N-(6-cyano-3-{2-[2-(2,4-dioxo-3,4-dihydropyrimidin-1(2H)-yl)ethoxy]phenoxy}-4-methylnaphthalen-1-yl)prop-2-enamide 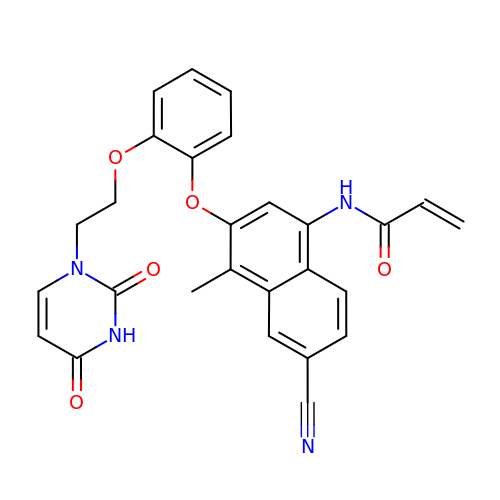| C27 H22 N4 O5 | FFULUQDOKSUESE-UHFFFAOYSA-N> MLKGKVAVVTGSTSGIGLGIATALAAQGADIVLNGFGDAAEIEKVRAGLAAQHGVKVLYDGADLSKGEAVRGLVDNAVRQMGRIDILVNNAGIQHTALIEDFPTEKWDAILALNLSAVFHGTAAALPHMKKQGFGRIINIASAHGLVASANKSAYVAAKHGVVGFTKVTALETAGQGITANAICPGWVRTPL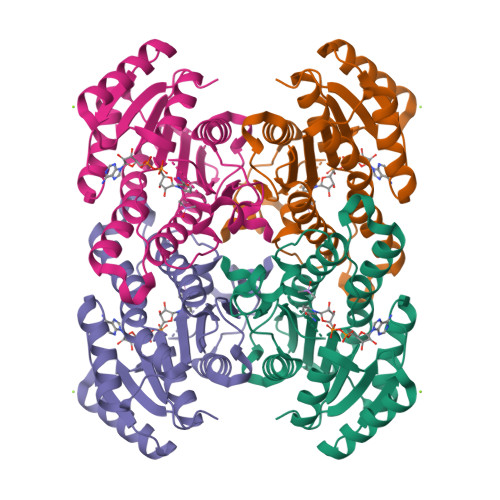VEKQISALAEKNGVDQETAARELLSEKQPSLQFVTPEQLGGTAVFLASDAAAQITGTTVSVDGGWTAR>MNRVSTVQQLTKRFSLGMLQGRGPLKLFMALVAFLRFLTIPPTAGILKRWGTIKKSKAINVLR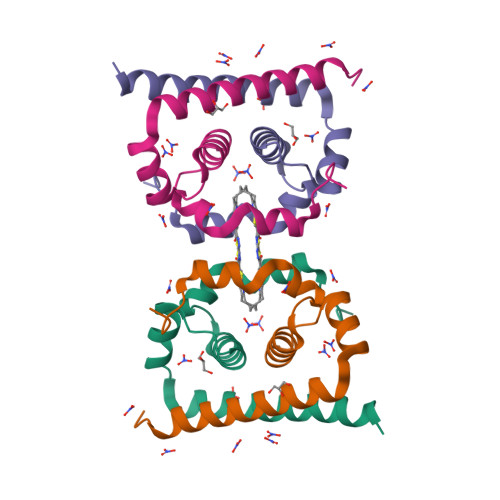GFRKEIGRMLNILNRRRR[2x]>AKMAFTLADRVTEEMLADKAALVVEVVEENYHAAPIVGIAVVNEHGRFFLRPETALADPQFVAWLGDETKKKSMFDSKRAAVALKWKGIELCGVSFDLLLAAYLLDPAQGVDDVAAAAKMKQ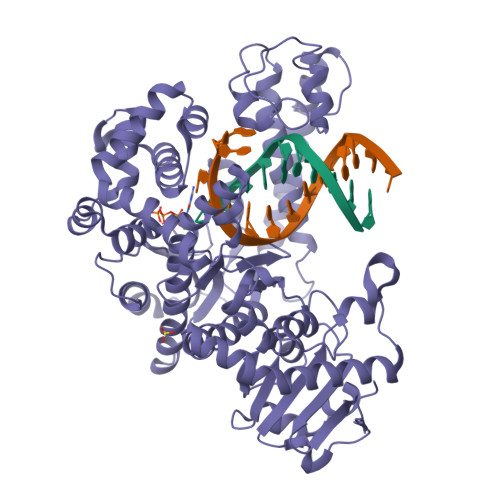YEAVRPDEAVYGKGAKRAVPDEPVLAEHLVRKAAAIWELERPFLDELRRNEQDRLLVELEQPLSSILAEMEFAGVKVDTKRLEQMGKELAEQLGTVEQRIYELAGQEFNINSPKQLGVILFEKLQLPVLKKTKTGYSTSADVLEKLAPYHEIVENILHYRQLGKLQSTYIEGLLKVVRPDTKKVHTIFNQALTQTGRLSSTEPNLQNIPIRLEEGRKIRQAFVPSESDWLIFAADYSQIELRVLAHIAEDDNLMEAFRRDLDIHTKTAMDIFQVSEDEVTPNMRRQAKAVNFGIVYGISDYGLAQNLNISRKEAAEFIERYFESFPGVKRYMENIVQEAKQKGYVTTLLHRRRYLPDITSRNFNVRSFAERMAMNTPIQGSAADIIKKAMIDLNARLKEERLQAHLLLQVHDELILEAPKEEMERLCRLVPEVMEQAVTLRVPLKVDYHYGSTWYDAK[2x]> MHHHHHHEQIGVNYGMDGNNLPSAGDVVSLMKKNNIGKMRIFGPNADVLRAFANSRIEVIVGVENKGLEAVASSQDSANGWVNDNIKPFYPSTNIKYIAVGNEVLEMPDNAQYVSFLVPAIKNIQTALENANLQNNIKVSTAHAMTVIGTSSPPSKGTFKDAVKDSMSSILQFLQDHGSPFMANVYPYFSYDGDRSIKLDYALFNPTPPVVDEGLSY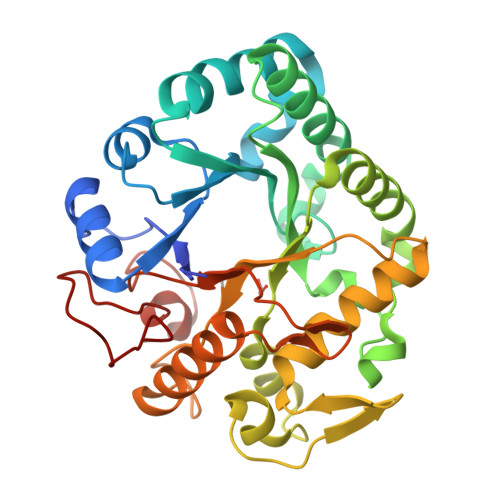TNLFDAMVDAVLSAMESLGHPNIPIVITESGWPSAGKDVATIENAQTYNNNLIKHVLSNAGTPKRPGSSIETYIFALFNENLKGPAEVEKHFGLFNPDEQPVYPVKFSLN>HEVYIKSTETGQYLRILPDGTVDGTRDRSDQHIQLQLSAESVGEVYIKSTETGQYLRILPDGTVDGTRDRSDQHIQLQLSAESVGEVYIKSTETGQYLRILPDGTVDGTRDRSDQHIQLQL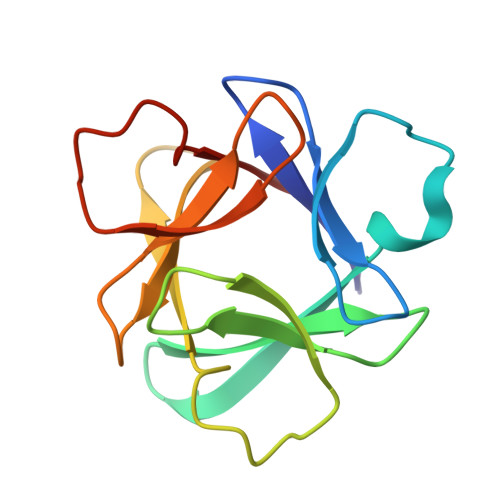SA[2x]The 9-1-1 DNA checkpoint clamp is loaded onto 5′-recessed DNA to activate the DNA damage checkpoint that arrests the cell cycle. Rad24 replaces Rfc1 and loads the DNA damage 9-1-1 ring onto DNA to signal DNA damage. Unlike RFC, which encircles DNA, Rad24 binds 5′-DNA on its surface, not inside the loader, and threads the 3′ ssDNA overhang into the 9-1-1 clamp from above the ring. Here we describe the first two structures of the Rad24-RFC–9-1-1 clamp bound to DNA and nucleotides, in closed and open conformations, at a resolution of 3.2 Å.

In one conformation the 9-1-1 ring is closed, but in the other the ring is wide open with a 27-Å gap. We found that Mec3 of the closed form undergoes a 45° in-plane rotation away from Ddc1 to generate the 27-Å gap in the open form of the 9-1-1 clamp. This is the largest gap observed so far in any DNA clamp-loader complex structure; the previously observed open clamp rings only have a gap of 10 Å or less that is too narrow for dsDNA to pass through. The third loop is hook-like, projecting from the Rad24 AAA+ domain, and interacts with Ddc1 of the 9-1-1 clamp in the closed state. This loop becomes disordered in the clamp open state. Therefore, we suggest that this Rad24 loop controls the 9-1-1 ring opening. In both closed and open 9-1-1 clamp states, the first four interfaces (Rad24:Rfc4, Rfc4:Rfc3, Rfc3:Rfc2 and Rfc2:Rfc5) are occupied by ATPγS and Mg2+, and an adenosine diphosphate (ADP) occupies the last interface between Rfc5 and the A′ subdomain of Rad24. This observation suggests that the 9-1-1 gate opening does not require ATP hydrolysis by Rad24-RFC.

> MDSTNLNKRPLLQYSLSSLGSQITKWSSSRPTSPVRKARSTENDFLSKQDTSSILPSINDDGGEQWYEKFKPNCLEQVAIHKRKLKDVQEALDAMFLPNAKHRILLLSGPSGCSKSTVIKELSKILVPKYRQNSNGTSFRSTPNEHKVTEFRGDCIVNDLPQMESFSEFLKGARYLVMSNLSLILIEDLPNVFHIDTRRRFQQLILQWLYSSEPLLPPLVICITECEIPENDNNYRKFGIDYTFSAETIMNKEILMHPRLKRIKFNPINSTLLKKHLKFICVQNMKMLKEKNKWNKRQEVIDYIAQETGDIRSAITTLQFWATSSGSLPISTRESTISYFHAIGKVIHGSHSTNNDNEMINNLFENSNNLLSKEDFKLGILENYNTFNKGEFSISDASSIVDCLSECDNMNGLPESNEYGLREVRKTFRNISKQGHNHGTVYFPREWKVRKLQNSFKVQAEDWLNVSLYKYNAVHSFRNITLEFGYYAPLIRKCQSYKKKYILYYLKNLPSGSSGPKQTMDKFSDIMKVENGIDVVDRIGGPIEALSVEDGLAPLMDNDSNNCDHLEDQKKERDRRLRMLIDQYERNVMMANDDLEDEETSFNDDPIVDSDSDNSNNIGNETFGRSDEDESLCEILSQRQPRKAPVISESLSDSDLEIL;> MSKTLSLQLPWVEKYRPQVLSDIVGNKETIDRLQQIAKDGNMPHMIISGMPGIGKTTSVHCLAHELLGRSYADGVLELNASDDRGIDVVRNQIKHFAQKKLHLPPGKHKIVILDEADSMTAGAQQALRRTMELYSNSTRFAFACNQSNKIIEPLQSRCAILRYSKLSDEDVLKRLLQIIKLEDVKYTNDGLEAIIFTAEGDMRQAINNLQSTVAGHGLVNADNVFKIVDSPHPLIVKKMLLASNLEDSIQILRTDLWKKGYSSIDIVTTSFRVTKNLAQVKESVRLEMIKEIGLTHMRILEGVGTYLQLASMLAKIHKLNNKA;> MSTSTEKRSKENLPWVEKYRPETLDEVYGQNEVITTVRKFVDEGKLPHLLFYGPPGTGKTSTIVALAREIYGKNYSNMVLELNASDDRGIDVVRNQIKDFASTRQIFSKGFKLIILDEADAMTNAAQNALRRVIERYTKNTRFCVLANYAHKLTPALLSRCTRFRFQPLPQEAIERRIANVLVHEKLKLSPNAEKALIELSNGDMRRVLNVLQSCKATLDNPDEDEISDDVIYECCGAPRPSDLKAVLKSILEDDWGTAHYTLNKVRSAKGLALIDLIEGIVKILEDYELQNEETRVHLLTKLADIEYSISKGGNDQIQGSAVIGAIKASFENETVKANV;> MFEGFGPNKKRKISKLAAEQSLAQQPWVEKYRPKNLDEVTAQDHAVTVLKKTLKSANLPHMLFYGPPGTGKTSTILALTKELYGPDLMKSRILELNASDERGISIVREKVKNFARLTVSKPSKHDLENYPCPPYKIIILDEADSMTADAQSALRRTMETYSGVTRFCLICNYVTRIIDPLASRCSKFRFKALDASNAIDRLRFISEQENVKCDDGVLERILDISAGDLRRGITLLQSASKGAQYLGDGKNITSTQVEELAGVVPHDILIEIVEKVKSGDFDEIKKYVNTFMKSGWSAASVVNQLHEYYITNDNFDTNFKNQISWLLFTTDSRLNNGTNEHIQLLNLLVKISQL;> MSLWVDKYRPKSLNALSHNEELTNFLKSLSDQPRDLPHLLLYGPNGTGKKTRCMALLESIFGPGVYRLKIDVRQFVTASNRKLELNVVSSPYHLEITPSDMGNNDRIVIQELLKEVAQMEQVDFQDSKDGLAHRYKCVIINEANSLTKDAQAALRRTMEKYSKNIRLIMVCDSMSPIIAPIKSRCLLIRCPAPSDSEISTILSDVVTNERIQLETKDILKRIAQASNGNLRVSLLMLESMALNNELALKSSSPIIKPDWIIVIHKLTRKIVKERSVNSLIECRAVLYDLLAHCIPANIILKELTFSLLDVETLNTTNKSSIIEYSSVFDERLSLGNKAIFHLEGFIAKVMCCLD;> MKLKLIVNGCEAPDDYKLLRTTINTVASLRKTAILRFNSERLTIISTPKSSLNSSNNGTILRGDTGQLWCTIPHDVFRLYTVISARELNTITMECNCDSLLSVFKRYDRVMNQGSSSNMTIKLQSCALGITFEEIVHTSGPNDAIVMNGGVDEHNGLPTTVGTGNLLASNKVIMHSFKVPVKLLFRAQDTRIQEPMINYIQLMMYKLPPISGEFGSAFHGFIRRVERYSNVNHIHLMGVKKKEHGNEGDDVELKIIVNELDWHLEICWNGPLDSVIQRQEGLTDNPSQNQHIDTDGRQEEGSLPIIEADKPMSSLYTNTRDREMEENIRYDEDLLRIEDSSIADTRGNIYTADTSGDTEFNDISVMVEKAEQESSSTHEVIIRCKDWKVCSKLYAAFEEVVLAISHDESCVFHCSLDRGSLEDSEDVEKPRERGQIIYYIARSKGL;> MRINSELANKFSASTVHLEHITTALSCLTPFGSKDDVLIFIDADGLSFVRENNHVIKIQLLLSRELFMSYSYRNETEDHMKLCVKINHILDSVSVMNRNSDDIVECTLSYDGHGSPFVLIFEDSFISERVEYSTYLIKDFDTNGLELDRERISFEAIIKGEALHSALKDLKEIGCKECYVYAKTEANDENVFALISKSQLGFSKIKLPSNRSILEKLQVFDGDSTTVIDGFAVIGFFDFTSFDKIRKSTKIASKVLFRMDVHGVLSVNILSQTDDVIITDTTRPSNNRPGSIRQLQLPKDYPGIVIEVCMLEKESIDEAAQTEIELLMETNELGNRNSFKKSTIRKRYGTDKGNETSNDNLLQLNGKKIKLPSEEENNKNRESEDEENHCKYPTKDIPIFF;> MSFKATITESGKQNIWFRAIYVLSTIQDDIKITVTTNELIAWSMNETDTTLCQVRFQKSFFEEYEFKPHEIVFGENGVQVIEDTYGNSHKLYSFRVNGRHLTTISRKPDGDGIKSFTIAVNNTSTCPESLANRLIVVIEMDSLIVKEYCPQFQPIKYDPIIINLKYKRRFLDVFGTAASDRNPQEPLDPKLLDVFTNTERELTSALFNEEVESDIRKRNQLTAADEINYICCNSTLLKNFLDNCNVNVTDEVKLEINVHRLSITAFTKAVYGKNNDLLRNALSMSNTISTLDLEHYCLFTTIEDEKQDKRSHSKRREHMKSIIFKLKDFKNFITIGPSWKTTQDGNDNISLWFCHPGDPILMQMQKPGVKLELVEVTDSNINDDILEGKFIKTAISGSKEEAGLKDNKESCESPLKSKTALKRENLPHSVAGTRNSPLKVSYLTPDNGSTVAKTYRNNTARKLFVEEQSQSTNYEQDKRFRQASSVHMNMNREQSFDIGTTHEVACPRNESNSLKRSIADICNETEDPTQQSTFAKRADTTVTWGKALPAADDEVSCSNIDRKGMLKKEKLKHMQGLLNSQNDTSNHKKQDNKEMEDGLGLTQVEKPRGIFD> MAYENLMLRPACPGNLSDTSTYNIDGACVAQGDIEFGSAVQVVGIVDGVKVVTALSDGGTPYGIAFRSQYEHLSGKILDGEVCNVVSHGRVWALTSLDEAPSLFSKLQFGSGGVVTGGSGYAGWTFAGGFVKHEDGYIIEVRVKQNAFIVPPPPPPVVLVESATITTDKESPQPNNVTIQCVANALPANATDKTGKWSIDATNIATVNPDSGLVTPVGGEVVGDFNITWTANDASKTTATI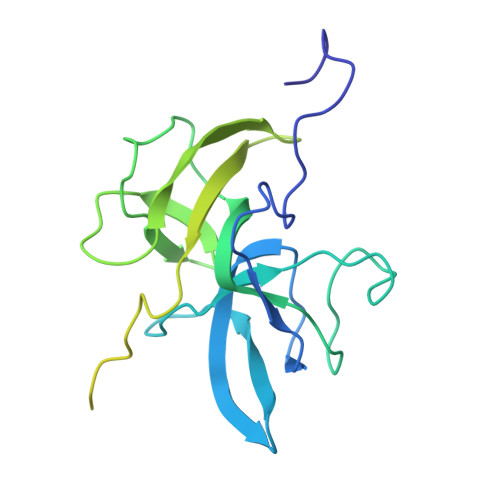AYRVEAVPTPEVDV5-(2-methylphenyl)-3H-1,2,4-triazole-3-thione 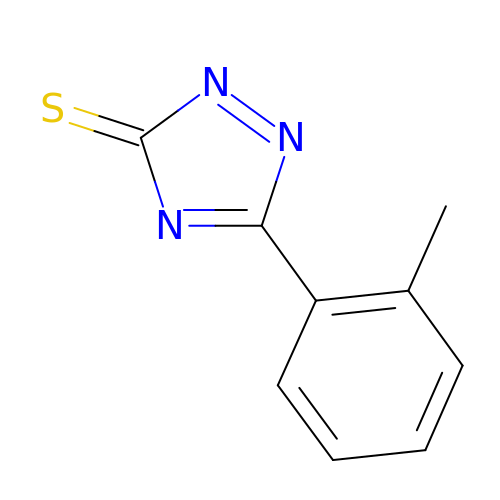| C9 H7 N3 S | DEADBTNDSDWXDC-UHFFFAOYSA-N>[2x]MGSDKIHHHHHHMAILNILEFPDPRLRTIAKPVEVVDDAVRQLIDDMFETMYEAPGIGLAATQVNVHKRIVVMDLSEDKSEPRVFINPEFEPLTEEMDQY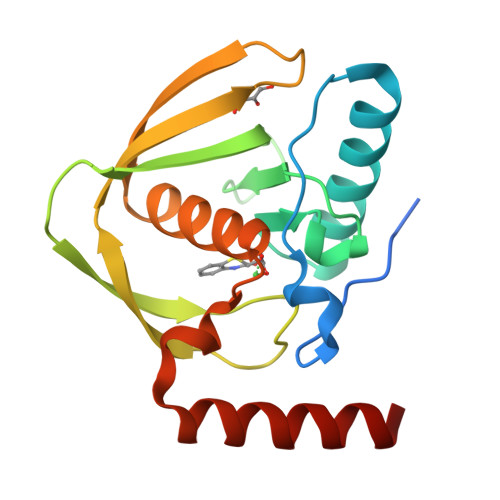QEGCLSVPGFYENVDRPQKVRIKALDRDGNPFEEVAEGLLAVCIQHECDHLNGKLFVDYLSTLKRDRIRKKLEKQHRQQA> SMQVERESISRLMQNYEKINVNEITRFSDFPLSKKTLKGLQEAQYRLVTEIQKQTIGLALQGKDVLGAAKTGSGKTLAFLVPVLEALYRLQWTSTDGLGVLIISPTRELAYQTFEVLRKVGKNHDFSAGLIIGGKDLKHEAERINNINILVCTPGRLLQHMDETVSFHATDLQMLVLDEADRILDMGFADTMNAVIENLPKKRQTLLFSATQTKSVKDLARLSLKNPEYVWVHEKA

DExD/H-box RNA helicases, from virus and bacteria to eukaryotes, play important roles in processes including ribosome biogenesis, RNA processing and folding, ribonucleoprotein (RNP) remodeling, RNA nuclear export, the regulation of RNA translation and transcription, and nonsense-mediated RNA decay. DExD/H-box proteins often contain accessory regulatory domains and localization modules, but their cores consist of two RecA-like domains joined by a short flexible linker. The N-terminal domain is commonly referred to as conserved domain-1, or DEAD-domain, and the C-terminal domain as conserved domain-2, or helicase domain. Both domains contribute to the binding site for RNA substrates and both contribute to ATP hydrolysis. We used X-ray crystallography to determine the structures of the DEAD-domains of DDX2A, DDX2B, DDX5, DDX10, DDX18, DDX20, DDX47, DDX52, and DDX53, as well as the helicase domains of DDX25 and DDX41.

DDX10 is probably involved in ribosome assembly. Fusion of the nucleoporin gene NUP98 with the DDX10 gene leads to the NUP98-DDX10 gene product. This fusion protein is involved in leukemogenesis. The 6th residue upstream of the conserved glutamine is an aromatic residue in most DEAD-box helicases. Its side chain stacks with the nucleotide base, stabilizing it in its position. Interestingly this residue is not conserved: While phenylalanine is most common, DDX10 has a tyrosine and DDX47 has a tryptophan in the corresponding position. In the crystal complexes with either ADP or AMP the loop closes up, resulting in a shift in Cα-atom positions by up to 3.5 Å between the ATP- and the AMP-states, or by up to 2.5 Å between the ADP- and the AMP-state. Thus the conformation of the P-loop is determined by the nucleotide phosphates, and longer phosphate tails result in a more open loop.>GTALAEMPKRKFTIDDFDIVRPLGKGKFGNVYLAREKQNKFIMALKVLFKSQLEKEGVEHQLRREIEIQSHLRHPNILRMYNYFHDRKRIYLMLEFAPRGELYKELQKHGRFDEQRSATFMEELADALHYCHERKVIHRDIKPENLLMGYKGELKIADFGWSVHAPSLRRRTMCGTLDYLPPEMIEGKTHDEKVDLWCAGVLCYEFLVGMPPFDSPSHTETHRRIVNVDLKFPPFLSDGSKDLISKLLRYHPPQRLPLKGVMEHPWVKANSRRVLPP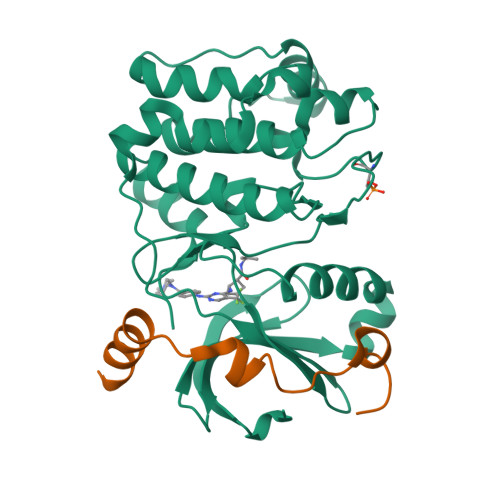VYQ[2x];>MDESQPRKPIPAWASGNLLTQAIRQQYYKPIDVDRMYGTIDSPKLEELFNKSKPRYFKR[2x]4-[2-AMINO-5-(4-HYDROXY-3-METHOXYPHENYL)PYRIDIN-3-YL]BENZAMIDE | C19 H17 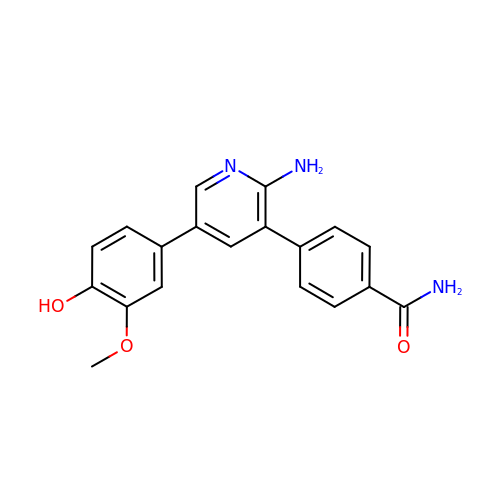N3 O3 | MGGHBVJICDPMQM-UHFFFAOYSA-N> MFGGQFGSFGAKPAATASPFGAPSAAPTTSLFGSTAPSSGFGGFGSTAQTTQPTTGGFGGFGGFGGATTTQQPAASPFGGGGTGGSGLFGSSAQTTTQQPGASPFGGGFGTTTTTTTQQPGASPFGGTGGGLFGSSAQTTTQQQGASPFGGFGGATTTQPSLLSGATGGFGGFGGSTTSGTQLGGGGGATSGAFGGSSSPFGGSGGATTSSPFGGGGGSFGATTQKQYGTPIPYQQTTIEGNTFVSISAMPQYNDRSFEELRFEDITHRKDIVYKTGGGSGGGNSLFGSTPTTQPSSPFGAQTTTQTTGGLFGGQTTTSPFGGQTSATPGSSLFGSTQPTQQQTSGGLFGSVQPTQQQAGGGLFGSMPSTGGSSLFGSTQPTQQQTGGAQPTQSLFGGQTQTTTSPFGSQTSTPFGQPQQTNTGSGLFGAQQTQQTNTGGGLFGAQPTQQTSGGGLFGTQPTSGTGLFGTSPTAGGTGLFGTTQPTSQGTGLFGTTQPTTQGTGLFGTSPTSGTGLFGSTPTSGTGLFGSTPTSGTGLFGSAQPPQNQQSQTSLFGNTGTGATNTGTGLFGSAQPSSNPGGGLFGSAQPSTTTGGLFGSNQPTAQPTTSLFGNTTGSVGGLGATPNITSGLFGSNPAQTGGLFGSTQPTTQTSLFGNTGSTGGLGAQNGGGLFGNLSQPTATAGQGLSGGLFGNLSQPTATAGQGLSSGGLFGNTLLGQPSTQGLSSALPTLGLGLMGGQPQQTQQLPQGSLMLQQTQQPLQQQPLQQQQQPLQQSTIQLNNQINSASPYFPISSPAPFATFVKDLTSTSKVVSPPSYTQRSLSHHGYIPKSTTKLVPRRGPNNVDLGFSVIQNQNGLFPIDKFITKHSKSLNINTTNETEDTLRSLNTKSSSLFNNNNNNNNNNNNRNVNTNVNDYQNNGLPSSSLYNSNINQLSNNNNNNNNIYNNNNNNNINNNNNNNNISTQFNLRNNQSSSDNLNNDKSLSSSSSNKSQQQQQKEQKEEQPPKPIKEKEFINPNAPKLTRDGYQCVPSIKELSKKTDKELSSVQGFTISRDGCGSIYFPGSTNLVALDLDDIVDIEPREVSVYK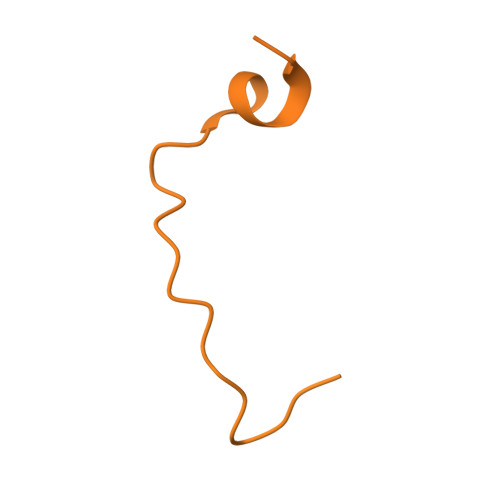DEETKPEIGYGLNRDAVVTLENCWPKNKNGEVVKEDGTILDKYENALKKVSAKSDCGFVSYSRSNGTWVFTVKHF> STPKKNISKGAVLHEKPMTVMVLTATEPFNYKEGKENMFHATVATESKYYRVKVFNMDLKEKFTENQFITISKYFNSSGILEINETATVSEAAPNQMFEVPKNIIRSAKETLKISKIKELDSGTLIYGVFAVEKKKVN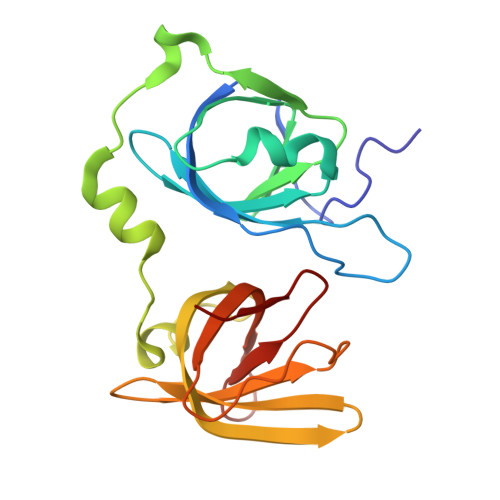DKSITFKIKDNEDNIKVVWDKEQHNINYEKGDKLQLFSFHLRKGNGKPILHSGNHSFIKGE>[4x]KKIFKPEELRQALMPTLEALYRQD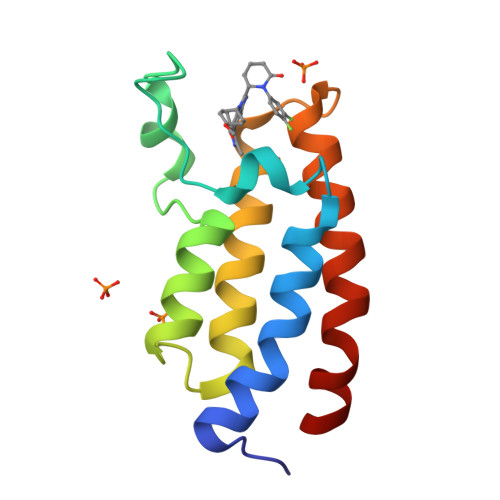PESLPFRQPVDPQLLGIPDYFDIVKNPMDLSTIKRKLDTGQYQEPWQYVDDVWLMFNNAWLYNRKTSRVYKFCSKLAEVFEQEIDPVMQSLG ethyl 7-imidazol-1-ylheptanoate | C12 H20 N2 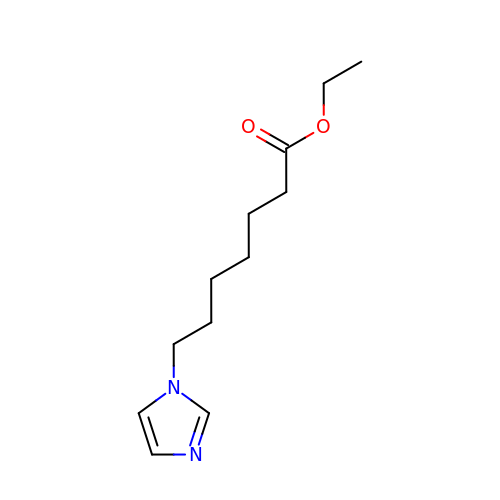O2 | IGQBGUMGRVQYDB-UHFFFAOYSA-N In this work, we exhaustively probe the ability of all 36 immobile HJ sequences to form DNA crystals in two different designed systems. Three separate self-assembling DNA crystal systems are described in this report: the “4 × 5” and “4 × 6” designs (collectively referred to as the 4 × N systems), and a third construct with a “scrambled” sequence variant of the 4 × 6 lattices. Self-assembly was mediated by three constituent oligonucleotides: (S1) containing four sequence repeats of either 5 or 6 bases; (S2) composed of 21 bases containing complementary regions to both (S1); and (S3) which forms the second junction crossover. The HJ serves as the fundamental component at the core of each unit, and the ultimate assembly of the full lattice is facilitated by the complementary 2-base sticky ends that tail each duplex.

Because the 4 × 6 system yielded R3 symmetry in 5 of 17 junctions, we considered whether the downstream sequences adjacent to the junction could play a role in crystallization efficiency, junction angle, and symmetry preference, or if the HJ alone was the singular determinant. To investigate this possibility, we designed “scrambled” sequences with targeted base substitutions, while maintaining GC content, along each “stem”. Contrary to the buffer preference observed with the native P32 crystals, the scrambled systems exhibited an exclusive preference towards low salt buffers, much like the native R3 crystals. Remarkably, only J1 and J2 retained the P32 symmetry, with all others yielding an R3 lattice. There appeared to be only a marginal difference in the average cell lengths in the R3 scramble crystals (a = b = 113.04 c = 51.10) relative to the native 4 × 6 sequences: the a, b axis trended ~2 Å shorter and c ~1.3 Å longer, whereas in the J1 and J2 cases, the crystals were in good agreement with the original 4 × 6 motif. The average angles of the R3 and P32 crystals were 61.00° (σ = 1.21) and 58.05° (σ = 1.39), respectively. Further, we observed modest improvements in resolution, reaching as high as 2.7 Å in J36. Notably, all junctions preventing crystallization compared to its original counterpart remained fatal and all relative cavity dimensions and volumes remained unperturbed. However, in the majority of the crystal structures reported here, the cacodylate anion indeed fits best into the electron density map of our X-ray structures, due to the presence of sodium cacodylate in the crystallization solution. A complete description of the comprehensive, experimental evidence for this arsenic has been described in our previous work. This seemingly counterintuitive result can be rationalized in several ways: First, the cacodylate could be stabilized at this site by hydrogen bonding and interactions with the solvent, both of which are known to provide stabilization for anionic binding even at regions with negative surface potentials.

> GAACGACACAGA;> CGGCGACTC;> TCTCCG;> TCGAGTCGGTGTCGT>SNAMAEICLITGTPGSGKTLKMVSMMANDEMFKPDENGIRRKVFTNIKGLKIPHTYIETDAKKLPKSTDEQLSAHDMYEWIKKPENIGSIVIVDEAQDVWPARSAGSKIPENVQWLNTHRHQGIDIFVLTQGPKLLDQNLRTLV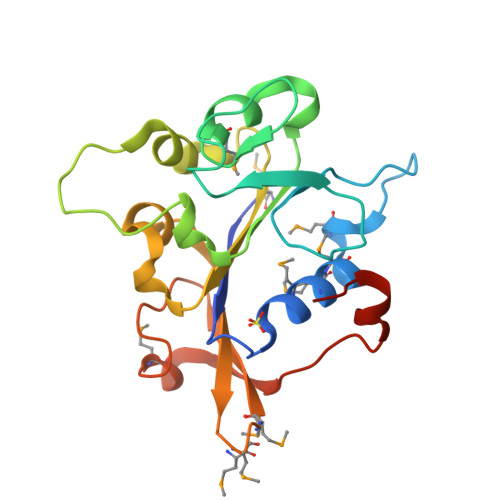RKHYHIASNKMGMRTLLEWKICADDPVKMASSAFSSIYTLDKKVYDLYESAEVHT[2x]> ML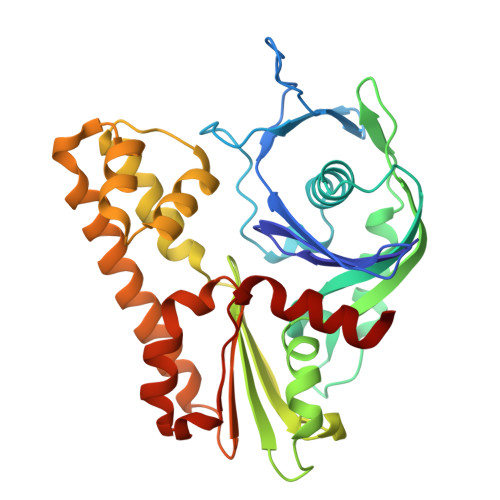VFIDDGSTNIKLQWQESDGTIKQHISPNSFKREWAVSFGDKKVFNYTLNGEQYSFDPISPDAVVTTNIAWQYSDVNVVAVHHALLTSGLPVSEVDIVCTLPLTEYYDRNNQPNTENIERKKANFRKKITLNGGDTFTIKDVKVMPESIPAGYEVLQELDEADSLLIIDLGGTTLDISQVMGKLSGISKIYGDSSLGVSLVTSAVKDALSLARTKGSSYLADDIIIHRKDNNYLKQRINDENKISIVTEAMNEALRKLEQRVLNTLNEFSGYTHVMVIGGGAELICDAVKKHTQIRDERFFKTNNSQYDLVNGMYLIGN>GPGYQDPERKLKILLDYSSKIANEKDLRNVLLFLTDLAKEIMEADRASIFLYDDQKKTLWTIVAHGVDRIEIDADKGIAGYVFRTGEILNIPDAYKDPRFDRDIDKRTGYRTRTILAVPLFDRKQNIIGVFQVINKLTNSVFTEEDIELLRHISLYASSTIENAILYEKLKKAHEDVIYRLSHATKFKDPETQNHIIRVGLYAEILAREAGLDEEDVELVKLAAPMHDIGKVGIPDRVLLKPGKLNDEEWEIMKKHTIYGYEILKGGDSRLLQIAADIAIEHHERWDGTGYPFGKKGEEISIYGRMTSISDVFDALTSDRPYKKAWDMDRTVRFFKEQKGKHFDPFLTDIFLKNIDQMFSIKRELRDED[2x]

Here we describe the first crystal structure of an enzymatically active HD‐GYP phosphodiesterase protein, PmGH from Persephonella marina EX‐H1, a thermophilic marine member of the Aquificales. PmGH comprises an HD‐GYP domain fused to a GAF domain. A remarkable feature of the structure of PmGH was the identification of a trinuclear Fe centre which is buried at the bottom of the cavity forming the c‐di‐GMP binding site.

The structure was solved by the single wavelength anomalous diffraction (SAD) technique using the anomalous signal from the bound iron. Anomalous diffraction difference maps showed all three metal sites to be occupied by iron atoms, with anomalous peak heights in excess of 40 σ separated by approximately 3.5 Å. The bond valence sum method was used to estimate the oxidation states of the three Fe ions which assigned the two peripheral sites as occupied by Fe(II) and the middle site by Fe(III). The tri‐iron centre delineates the floor of the open chela with the two peripheral metal sites being in close proximity to Y285 of the GYP motif on one side (the G‐site) and H221 of the HD motif on the other side (the H‐site). The middle iron binding site (M‐site) is sandwiched between the G‐ and H‐sites with Fe‐Fe bond distances of 3.40 Å and 3.67 Å respectively. All three metals are octahedrally co‐ordinated. In PmGH the HD‐GYP domain conserved residues E185, H189, H221, D222, H250, H276, H277 and D305 contribute to ligand binding with the metal co‐ordination sphere completed by succinate and imidazole bound from the crystallization buffer as well as two solvent molecules which bridge the G‐M and M‐H metal pairs. Both pairs of Fe sites, G‐M and M‐H, are triply bridged: the G‐M pair by the carboxylate groups of D222 and a succinate from the crystallization buffer in a bidentate fashion and by a monodentate bridged solvent molecule; whereas the M‐H pair is bidentately co‐ordinated by the carboxylate groups of E185 and a second succinate ion and by another monodentate bridged solvent molecule. Analysis of metal‐ligand bond lengths for the bridging solvent molecules is consistent with the bridging ligand being a hydroxide ion. PmGH presents an accessible and far larger binding cavity than is the case for Bd1817 where the active site is capped by a ‘lid’ formed by loops corresponding to L7/8 and L10/11 in PmGH.ALENDRONATE | C4 H13 N O7 P2 | 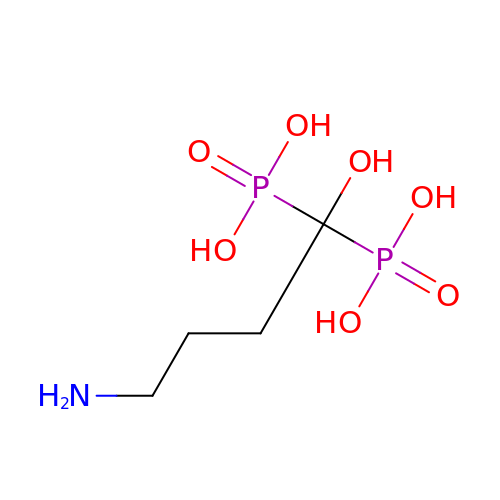OGSPWJRAVKPPFI-UHFFFAOYSA-N methyl cis-4-({[3-(thiophen-3-yl)benzyl]amino}methyl)cyclohexanecarboxylate | C20 H25 N O2 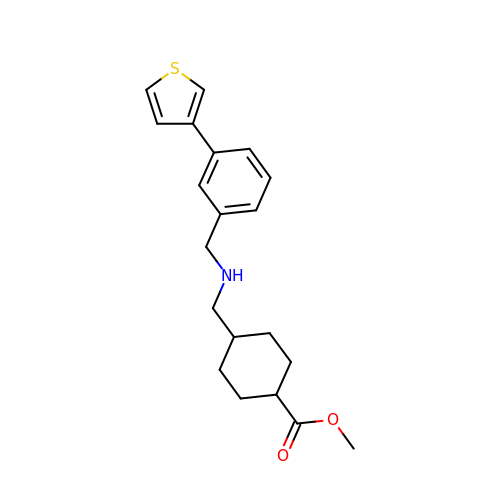S | YJJNZSNCUYMDTL-WOVMCDHWSA-N>MIRNRLSELLSERGLKISRVAKDVKIARSSLTSMAQNDSEMIRYDAIDKLCSYLHISPSEFFEHNPINFDFTFDEEPNYKINDVFEGFEVTANITHAFSIENFDFEILVDVELDNRQKLNFDLDVSYKETEKITNSQHRFIFTIKNEDENIGLKKYVDSLSAGLKNLLFKKINQKLSGYVSEIIVKNIDDIEELFPNKGEKSTTLHKEILQTDSRLSSDIFKEYLEHHHHHH[8x]

To parasitize a phage, the SaPIs employ a transcriptional repressor, Stl, which in addition to repressing the SaPI genes, senses an active phage infection by binding to the phage-encoded anti-repressor protein. Here, we show that the phage satellite SaPI2, which does not encode orthodox anti-phage defense systems, provides antiviral immunity mediated by Stl2, the SaPI2-encoded transcriptional repressor. Stl2 targets and inhibits phage-encoded HRs, including Sak and Sak4, two HRs from the Rad52-like and Rad51-like superfamilies. Here we have focused on two recombinases, an annealase called Sak, and a recombinase called Sak4, belonging to the Rad52-like and Rad51-like superfamilies respectively.

Investigating Stl2’s oligomeric state by mass photometry showed two peaks, one corresponding to the dimeric form (54 kDa) and a second peak of 626 kDa, indicating that Stl2 displayed distinct oligomeric states in solution. To further analyze the oligomeric state of Stl2 in solution we solved the apo Stl2 structure by cryo-EM. Surprisingly, the micrographs showed circular structures as well as long curved filaments, highlighting Stl2’s intrinsic tendency to oligomerize mimicking its target’s architecture. We generated a cryo-EM map of the undecamer state with C11 symmetry and discovered that the circles were composed by 11, 12, and 13 dimers of Stl2. We extracted particles with a smaller box size so that three complete Stl2 dimers were resolved imposing D1 symmetry at an overall 3.7 Å resolution. Notably, at the interfaces of monomer-monomer and dimer-dimer contacts, the local resolution improved to 2.5 Å. The structure of the dimer displays a peculiar butterfly shape, where the N-terminal domain (NTD) and the C-terminal domain (CTD) are the body and the wings of the butterfly respectively. The dimer-dimer interface corresponds to a patch of the antiparallel β-sheet present in the CTD and the α-helix 2 present in the NTD. We first analyzed these two mutants by mass photometry and confirmed that they displayed only one peak corresponding to the dimeric state, indicating that they had lost their ability to form circles/filaments of dimers. The Stl2 apo structure therefore suggests that its ability to oligomerize into large multimeric structures is the basis for its promiscuity in targeting phage-encoded HRs from structurally divergent superfamilies.The best-characterised SAAT, antigen 43 (Ag43), is a protein that contributes to cell aggregation and biofilm formation in commensal Escherichia coli K-12 as well as in major pathotypes including enterohemorrhagic E. coli (EHEC) and uropathogenic E. coli (UPEC). Ag43 possesses a modular domain organisation that is common throughout the ATs, which encompasses an N-terminal signal sequence that directs the secretion of the protein across the inner membrane, a passenger (α) domain that is responsible for the function of the protein, and a C-terminal translocator (β) domain that facilitates the translocation of the functional α-domain to the cell surface. After translocation, the Ag43 α-domain (α43) is cleaved but remains attached to the cell via non-covalent interactions. Similar to α43a 13, the α-domain of all three Ag43 variants folds into an L-shaped right-handed three-stranded β-helix, with each turn of the β-spine comprising three β-strands linked by loop regions.

Crystals of α43_UTI89 and α43b belong to the C2 and P21221 space groups, respectively, and each contained one molecule per asymmetric unit. Although α43a and α43b are similar in size, the α43b crystallised in this work is truncated and lacks the bottom section of the L-shaped β-helix. The α43b truncation occurred during recombinant protein purification with cleavage occurring at residue 415, possibly by a protease mechanism that remains to be defined. Although Ag43a and Ag43b share 86% sequence identity in their respective α-domains, these proteins differ significantly in their aggregation profiles. Unlike α43a, α43b did not crystallise in its dimeric form. However, given the similarity between α43a and α43b, we superimposed two α43b structures on the α43a–α43a functional dimer13 to infer the potential α43b dimerisation interface, which consisted of two interfaces encompassing a total of 14 hydrogen bonds. To confirm if this interface was indeed responsible for the aggregation phenotype of Ag43b, we mutated residues D29, N60, R62, D79 and S95 to glycine (Ag43bmt) and tested an MS528 strain expressing this mutant protein in aggregation assays. Substitution of these five interface residues completely abolished the ability of Ag43b to mediate cell–cell aggregation compared with Ag43b WT, confirming the predicted mode of self-association. Although α43b–α43b trans-dimers are stabilised by a double-interface, this interface consists of only 14 hydrogen bonds. This reduced bonding network results in Ag43b-expressing cells displaying a reduced aggregation profile comparable to that of Ag43UTI89.

> SNAADSVVPAGETVNGGTLINHDRQFVSGTADGMTVSTGLELGADSDNNTGGQQIARGGTARNTRVTANGLQDVMAGGSTSDTVISTGGGQNLRGKASGTVLNDGDQWIHAGGRASGTVINQDGYQTIKHGGLVTGTIVNTGAEGGPDSENVSTGQMVGGIAESTTINKNGRQVIWSSGIARDTLIYTGGDQTVHGEAHNTRLEGGNQYVHKYGLALNTVINEGGWQVVKAGGTAGNTTINQNGELRVHAGGEASDVTQNTGGALVTSTAATVTGTNRLGAFSVVEGKADNVVLENGGRLDVLSGHTATRTLVDDGGTLDVRNGGTATAVSMGNGGVLLADSGAAVSGTRSDGTAFRIGGGQADALM> GSHMEEKRLSAKKGLPPGTLVYTGKYREDFEIEVMNYSIEEFREFKTTDVESVLPFRDSSTPTWINITGIHRTDVVQRVGEFFGTHPLVLEDILNVHQRPKVEFFENYVFIVLKMFTYDKNLHELESEQVSLILTKNCVLMFQEKIGDVFDPVRERIRYNRGIIRKKRADYLLYSLIDALVDDYFVLLEKIDDEIDVLEEEVLERPEKETVQRTHQLKRNLVELRKTIWPLREVLSSLYRDVPPLIEKETVPYFRDVYDHTIQ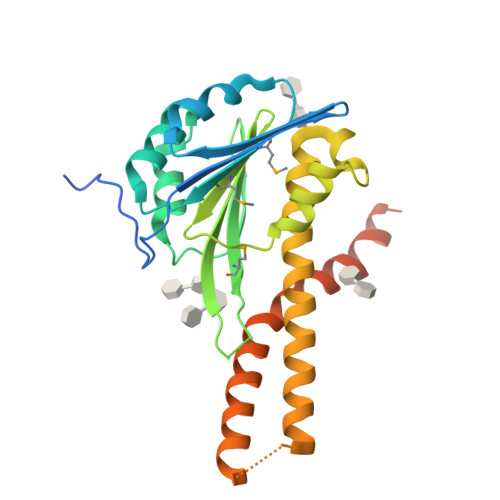IADTVE>[3x]MFIYYKRTKQGSTEQWFVIGGKRIYLPTMTYVNEANDLIKRYGGNTNVTTYNHDNFGLKMMEAALPQVKV;> MVKLNDVLSYVNGLVGKGVDADGWYGTQCMDLTVDVMQRFFGWRPYGNAIALVDQPLPAGFQRIRTTSSTQIKAGDVMIWGLGYYAQYGHTGIATEDGRADGTFVSVDQNWINPSLEVGSPAAAIHHNMDGVWGVIRPPYEAASTPKP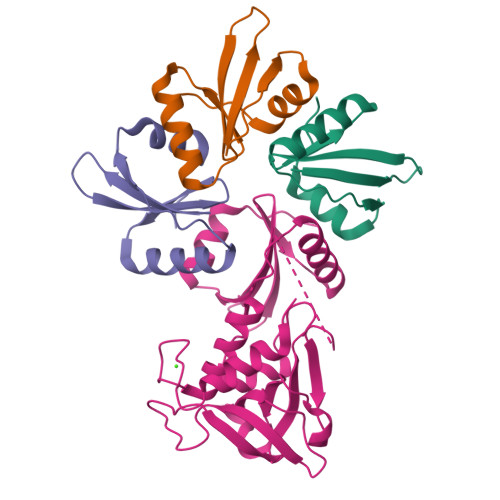PAPKPDKPNLGQFKGDDDIMFIYYKRTKQGSTEQWFVIGGKRIYLPTMTYVNEANDLIKRYGGNTNVTTYNHDNFGLKMMEAALPQVKV> MKDNSTSAVSSWLGYKIQEYRLTQRLLEANNSSCIGFEILDDLEEHTGSTSTFEQDKISTTGRNIVSNHSKDLWKTLSNWMDLIDSGEIDVDNTIFLLFTNKRCHSEVLQLLSTSQATEEASKAFDEILKIVSHPSPSIANYLNNFSKSKTDACRLISKFTYIYGSGSAPHDLRESYKLHRLGALEEHLDEIMYEILGWVSDVLTLAAEKRQPTIVRAKDFGARLGEIESKYRQKTILNYFCNRSSESEDVQNTIKDAPNYIKQLNLINVDDSELEEAAIANLETKDAVVEWTLNGDVQDYSYRYYQRELRRCWGIQKQKIHLDFNGRPETEVGQRLYIECLNNVTRYYLENKKVGDFFAHGTLHSMADKLTIGWHPEFDKKLGDPDA;>MFFQIEKVVLWSKEAKHKPRVIEFALNKVNLITGSSKSGKSSLIPIIDYCLGSSKCSIPVNTIRDTTAWYGVQIKTKHSRLLIARRDPSNQLSTSNAFFVEAENIEIPQNIEKHNVNIDTVKNRLNEISGVSNISFDFYDTGRIDKKRTSTRDLSAFNYQPQNIIANPNALFYKTDSFEHKSKLVTILPYVLGALSNTDIENQHRIKNLEEEYRKVERRLLKLKRQNEDWLSSAQAYVIKAMELGLVNSDKDIYQLKPERLLNVLKNIATKEIDYSTSAANIKYASEQEAEITKRSRDISNNLAKVKSRLQNINSMNRLANTHSDASRLKRERLSLSKWLLTQNDINSSLFSEPNEIRSLVLEPLARAFSNLEAELEVPIHVQGALSREKIYLEGELTRLASEMKDVNTQLKILRGNKRKLGYDAFSVGKFVGEVEKALSLMGESESESELSKEYKRLKKELSVLRLKIDPREFERKTKLQLAKVNKLASDWLPHLDTENPNAPISLHEKELTITVNSSGREDYLWEIGSGANWLSYHVAITLALHQHFSSLEASPVPNYIIYDQPSQVYFPSKLRHQATPEEDELALLEQDEDIVQVKKIFEAFNGAIEKTKDNLQIIVLDHAPSTLVKSIPKGHLVEEWRNGIKLIPLDWL[2x];> MIKNLEIQMLKPENNLEKEAWEINNPAMCSYMLWIATLAYYQKQKEPIHPSRLFCLFPFILYSDTRNVLLSSKGSLKSYLAKFSNSKAISGDIPLSIHFRIDIQKNKTLDALIVAFDSGLLVIDSDSGLIKPNVSIKPLPNSKLTD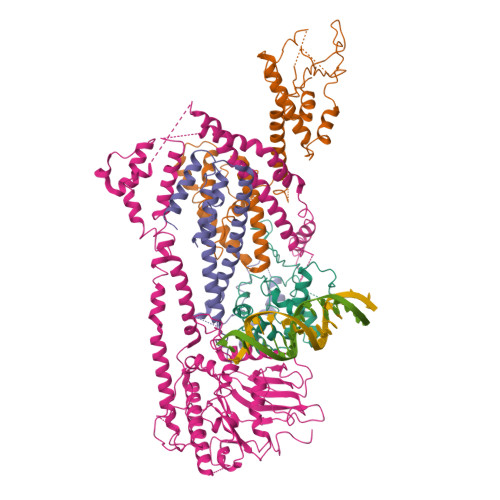TIKELVYCSTKIGRWLSEMTNQDLARDLKVIF> GHMMVKIMPNLPGLYFLQ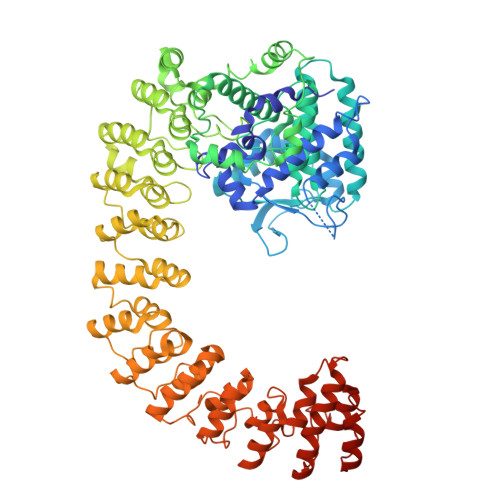AYPSEEIWRLFVDGRFWSKENGWRGYESREPGSLNAALESLCSIALQVEKSGEEFELSVDLIKRIHKKSGKKVEELQEKNPGELRTDEPVSFCIPAGRASIKGIEEFLSLVFLTEGGAEFGPGKAGPFGPRFDKNYFKNLNPEQIPDLAKQIYFDMSKYGHSNTNHFYLAVMKNVDVYLEKITQSYNKEIKTAETLDEKLKIIVKHIRMYEVLHPFRDANGRTFVNNLLNILLMQQGLPPATFYEPNVFDLYSAEELVVVVKEAIFNTVEIIEQSKRKTPITLYGYHSSLEEQTKFRDMLDSPSYEKIKHMDFSDLNPEKLHLKTQKCLSSLNEQYPLHRGAIYLSDPGEIKLLLSNRNESQINQQIEQGAPPIYVGKTPAHLAVISGNMAMLDELIAKKADLSLQDYDGKTALHYAAECGNMQIMGKILKVVLSQEDAIKVLNIKDNHGKTAFHYAAEFGTPELISALTTTEVIQINEPDNSGSSAITLAYKNHKLKIFDELLNSGADISDELLDAIWARKDKETLGKIIAKNEKILLNKEAFRIAISLGSVSLVKKFLRAGVDIDIPLTKDKATPLMLSINSGNPKLVSYLLKKGANTRLTDTSGNSVLHYVFYSKAENREALANIITEKDKKLINQPNANGNPPLYNAVVVNDLKMATILLEMGARVDFEDRLGNNILHSAMRRCDLPIILDIVKKDSTLLHKRNSERRNPFHQALHEMHTFPSSKETEEIHFMNLSDLLLKEGVDLNKKDIKGKTILDIALSKQYFHLCVKLMKAGAHTNI> VNMEYTKEKKVGEGTYAVVYLGCQHSTGRKIAIKEIKTSEFKDGLDMSAIREVKYLQEMQHPNVIELIDIFMAYDNLNLVLEFLPTDLEVVIKDKSILFTPADIKAWMLMTLRGVYHCHRNFILHRDLKPNNLLFSPDGQIKVADFGLARAIPAPHEILTSNVVTRWYRAPELLFGAKHYTSAIDIWSVGVIFAELMLRIPYLPGQNDVDQMEVTFRALGTPTDRDWPEVSSFMTYNKLQIYPPPSRDELRKRFIAASEYALDFMCGMLTMNPQKRWTAVQCLESDYFKELPPPSDPSSIK;> DLYRHSSQYRMWSYTKDQLQEKRVDTNARAIAYIEENLLKFREAHNLTEEEIKVLEAKAIPLTMEEELDLVNFYAKKVQVIAQHLNLPTEVVATAISFFRRFFLENSVMQIDPKSIVHTTIFLACKSENYFISVDSFAQKAKSTRDSVLKFEFKLLESLKFSLLNHH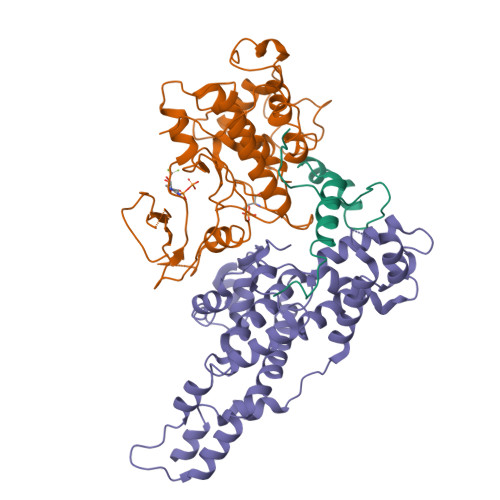PYKPLHGFFLDIQNVLYGKVDLNYMGQIYDRCKKRITAALLTDVVYFYTPPQITLATLLIEDEALVTRYLETKFPSREGSQESVPGNEKEEPQNDASTTEKNKEKSTESEEYSIDSAKLLTIIRECKSIIEDCKPPSTEEAKKIAAKNYYCQNPSTL;> PFNGDREAHPPFTLKGSVYNDPFIKDLEHRKEFIASGFNTNYAYERVLTEAFMGLGCVISEEL> ALVFFAE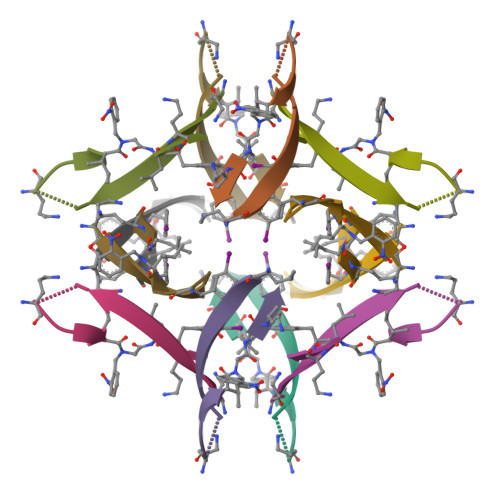DAAIIXLAV>MKQTVAAYIAKTLESAGVKRIWGVTGDSLNGLSDSLNRMGTI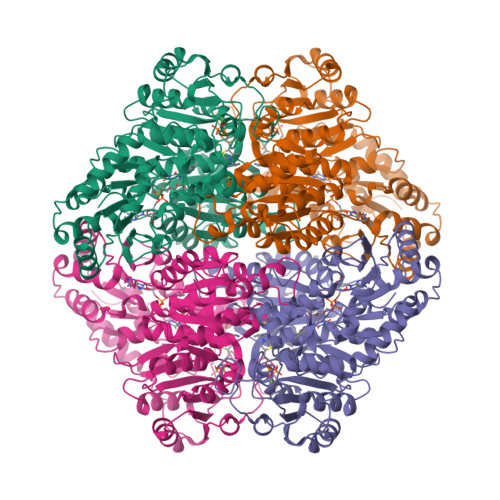EWMSTRHEEVAAFAAGAEAQLSGELAVCAGSCGPGNLHLINGLFDCHRNHVPVLAIAAHIPSSEIGSGYFQETHPQELFRECSHYCELVSSPEQIPQVLAIAMRKAVLNRGVSVVVLPGDVALKPAPEGATMHWYHAPQPVVTPEEEELRKLAQLLRYSSNIALMCGSGCAGAHKELVEFAGKIKAPIVHALRGKEHVEYDNPYDVGMTGLIGFSSGFHTMMNADTLVLLGTQFPYRAFYPTDAKIIQIDINPASIGAHSKVDMALVGDIKSTLRALLPLVEEKADRKFLDKALEDYRDARKGLDDLAKPSEKAIHPQYLAQQISHFAADDAIFTCDVGTPTVWAARYLKMNGKRRLLGSFNHGSMANAMPQALGAQATEPERQVVAMCGDGGFSMLMGDFLSVVQMKLPVKIVVFNNSVLGFVAMEMKAGGYLTDGTELHDTNFARIAEACGITGIRVEKASEVDEALQRAFSIDGPVLVDVVVAKEELAIPPQIKLEQAKGFSLYMLRAIISGRGDEVIELAKTNWLR[2x]>SMLPREKLNPPTPSIYLESKRDAFSPVLLQFCTDPRNPITVIRGLAGSLRLNLGLFSTKTLVEASGEHTVEVRTQVQQPSDENWDLTGTRQIWPCESSRSHTTIAKYAQYQASSFQESLQEEKESEDEESEEPDSTTGTPPSSAPDPKNHHIIKFGTNIDLSDAKRWKPQLQELLKLPAFMRVTSTGNMLSHVGHTILGMNTVQLYMKVPGSRTPGHQENNNFCSVNINIGPGDCEWFAVHEHYWETISAFCDRHGVDYLTGSWWPILDDLYASNIPVYRFVQRPGDLVWINAGTVHWVQAT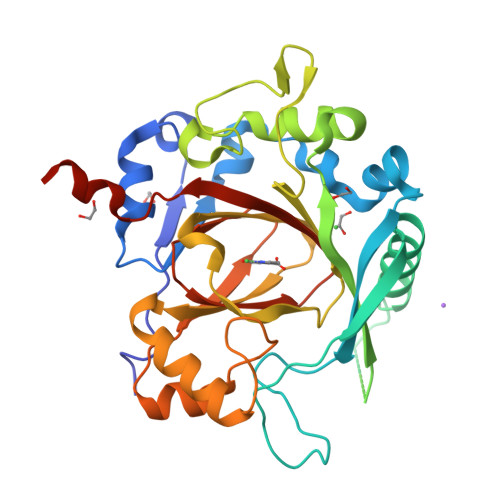GWCNNIAWNVGPLTAYQYQLALERYEWNEV[2x]Lassa virus (LASV) is an enveloped, ambi-sense, bi-segmented RNA virus endemic throughout Western Africa and is the most lethal of all known Old World arenaviruses. GP is synthesized as an inactive precursor preGPC, which is co-translationally cleaved by signal peptidase into GPC and the stable signal peptide (SSP). Post-translational maturation cleavage of GPC by host protease SKI-1/S1P yields the receptor-binding subunit GP1 and the membrane-spanning fusion subunit GP2. SSP is not only critical by functioning as a trans-acting maturation factor, but also associates with the GP2 subunit, resulting in a tripartite mature GP complex on the viral surface.

To account for possible effects of chemical fixation, we exploited a previously reported stable cell line expressing non-infectious virus-like particles (VLPs) displaying the full-length LASV GP but lacking the Z. Similar to the fixed virions, VLPs purified from cell culture supernatants were covered with GP spikes (VLP pH 7). To study GP conformation at endosomal pH, we determined the VLP-derived GP structure at pH 5.2 (pH 5, and S1 Fig VLP pH 5). The structure was resolved at 16-Å resolution and revealed conformational differences when compared to the same structure at pH 7.3 (pH 7). These can be attributed to a conformational difference at the membrane-proximal legs and a slight opening up of the spike, creating crevices at the top of the spike between the GP subunits. To localize the GP1 and determine its orientation relative to the LAMP1 binding site, we used volumetric correlation to fit the GP1 crystal structure into our GP reconstruction. As the GP1 has been crystallized at pH 5 and acidic pH has been suggested to have an effect on GP1 conformation, we used our GP structure derived from VLPs at pH 5 for fitting. The fitting was unambiguous (cross-correlation coefficient 0.86) and placed the GP1 structure to the membrane distal part of the spike. Interestingly, the triad of histidines that has been indicated in LAMP1 binding points towards the crevice between GP1 subunits, the putative LAMP1 binding side. The histidines may act as a pH sensor opening up the spike at pH 5 to create a binding site for LAMP1, but further studies are needed to test this hypothesis. Here, the membrane-distal GP1 remained bound to the membrane-anchored GP2 at pH 5.0, possibly providing an analogous shielding function and at the same time creating a binding site for the intra-cellular receptor LAMP1.

> SHHHHHHGGMETLNMTMPLSCTKNNSHHYIMVGNETGLELTLTNTSIINHKFCNLSDAHKKNLYDHALMSIISTFHLSIPNFNQYEAMSCDFNGGKISVQYNLSHSYAGDAANHCGTVANGVLQTFMRMAWGGSYIALDSGRGNWDCIMTSYQYLIIQNTTWEDHCQFSRPS> NMNIEEFTSGLAEKGISLSPRQLEQFELYYDMLVEWNEKINLTSITEKKEVYLKHFYDSITAAFYVDFNQVNTICDVGAGAGFPSLPIKICFPHLHVTIVDSLNKRITF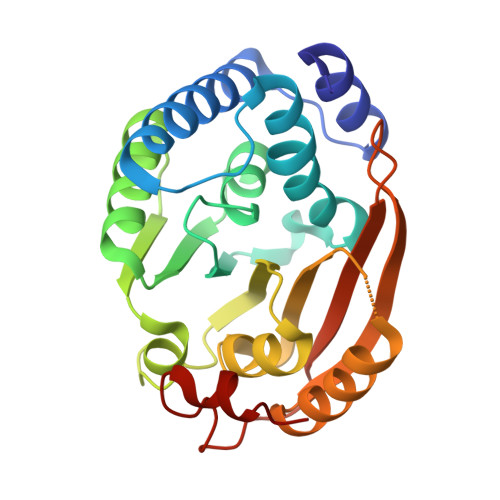LEKLSEALQLENTTFCHDRAETFGQRKDVRESYDIVTARAVARLSVLSELCLPLVKKNGLFVALKAASAEEELNAGKKAITTLGGELENIHSFKLPIEESDRNIMVIRKIKNTPKKYPRKPGTPNKSPIEG4-Maleylacetoacetic acid | C8 H8 O6 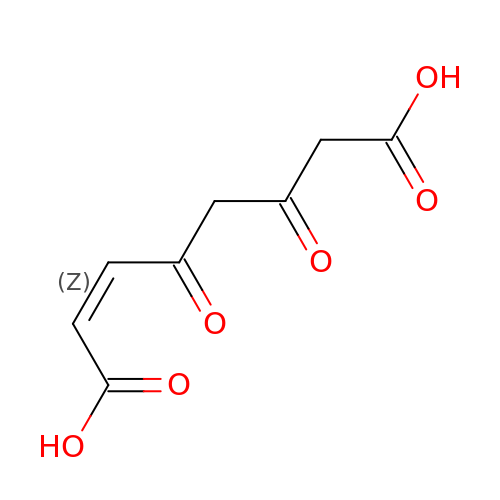| GACSIVHAIFQKTC-UHFFFAOYSA-N> VPACTVSNTTVDWQDVEIQTLSQNGNHEKEFTVNMRCPYNLGTMKVTITATNTYNNAILVQNTSNTSSDGLLVYLYNSNAGNIGTAITLGTPFTPGKITGNNADK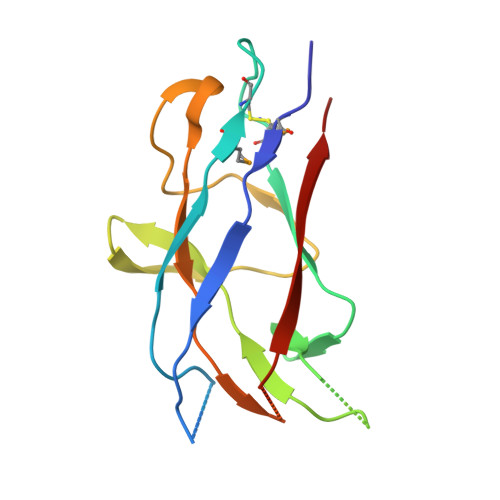TISLHAKLGYKGNMQNLIAGPFSATATLVASYS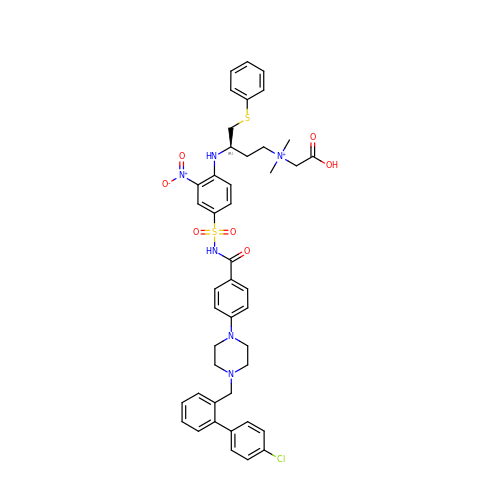[(3~{R})-3-[[4-[[4-[4-[[2-(4-chlorophenyl)phenyl]methyl]piperazin-1-yl]phenyl]carbonylsulfamoyl]-2-nitro-phenyl]amino]-4-phenylsulfanyl-butyl]-(2-hydroxy-2-oxoethyl)-dimethyl-azanium | C44 H48 Cl N6 O7 S2 | RWBVZZCFXRVCAC-PSXMRANNSA-O N-(tert-butoxycarbonyl)-L-alpha-glutamyl-N-[(1R)-1-(carboxycarbonyl)-3,3-difluoropropyl]-L-leucinamide | C21 H33 F2 N3 O9 | 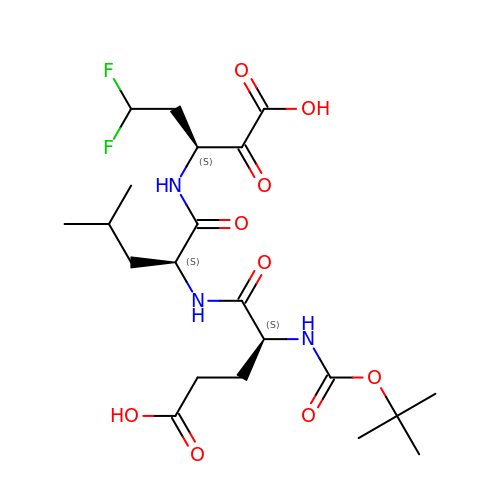WXVMZATZAOHPFR-AVGNSLFASA-N>SKPKQPPDASPANLLTSLVRAHLDSGPSTAKLDYSKFQELVLPHFGKEDAGDVQQFYDLLSGSLEVIRKWAEKIPGFAELSPADQDLLLESAFLELFILRLAYRSKPGEGKLIFCSGLVLHRLQCARGFGDWIDSILAFSRSLHSLLVDVPAFACLSALVLITDRHGLQEPRRVEELQNRIASCLKEHVAAVAGEPQPASCLSRLLGKLPELR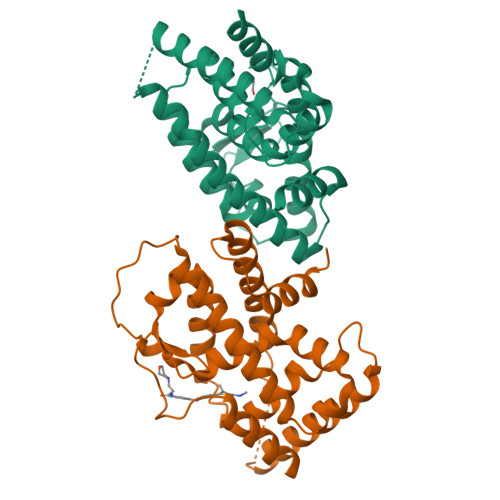TLCTQGLQRIFYLKLEDLVPPPPIIDKIFMDTLPF[2x]>MSVEKIPGYTYGETENRAPFNLEDLKLLKEAVMFTAEDEEYIQKAGEVLEDQVEEILDTWAGFVGSHPHLLYYFTSPDGTPNEKYLAAVRKRFSRWILDTSNRSYDQAWLDYQYEIGLRHHRTKKNQTDNVESVPNIGYRYLVAFIYPITATMKPFLARKGHTPEEVEKMYQA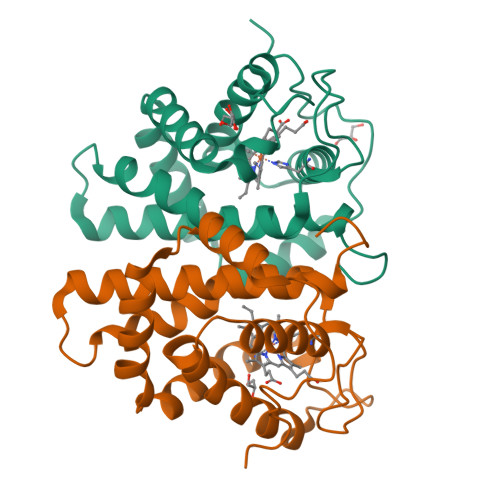WFKATTLQVALWSYPYVKYGDF[2x]> SFSNFPISEETIKLLKGRGVTFLFPIQAKTFHHVYSGKDLIAQARTG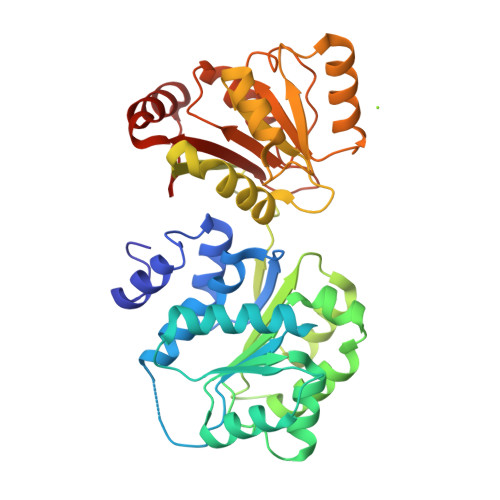TGKTFSFAIPLIEKLHGELQDRKRGRAPQVLVLAPTRELANQVSKDFSDITKKLSVACFYGGTPYGGQFERMRNGIDILVGTPGRIKDHIQNGKLDLTKLKHVVLDEVDQMLDMGFADQVEEILSVAYKKDSEDNPQTLLFSATCPHWVFNVAKKYMKSTYEQVDLIKTAITVEHLAIKCHWTQRAAVIGDVIRVYSGHQGRTIIFCETKKEAQELSQNSAIKQDAQSLHGDIPQKQREITLKGFRNGSFGVLVATNVAARGLDIPEVDLVIQSSPPKDVESYIHRSGRTGRAGRTGVCICFYQHKEEYQLVQVEQKAGIKFKRI>[2x]DADLDKQVNTAGAWPIATGGYYSQHNSPLAQINKSNVKNVKAAWSFSTGVLNGHEGAPLVIGDMMYVHSAFPNNTYALNLNDPGKIVWQHKPKQDASTKAVMCCDVVDRGLAYGAGQIVKKQANGHLLALDAKTGKINWEVEVCDPKVGSTLTQAPFVAKDTVLMGCSGAELGVRGAVNAFDLKTGELKWRAFATGSDDSVRLAKDFNSANPHYGQFGLGTKTWEGDAWKIGGGTNWGWYAYDPKLNLFYYGSGNPAPWNETMRPGDNKWTMTIWGRDLDTGMAKWGYQKTPHDEWDFAGVNQ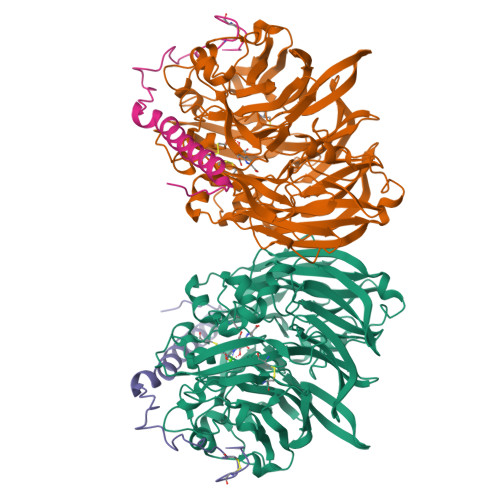MVLTDQPVNGKMTPLLSHIDRNGILYTLNRENGNLIVAEKVDPAVNVFKKVDLKTGTPVRDPEFATRMDHKGTNICPSAMGFHNQGVDSYDPESRTLYAGLNHICMDWEPFMLPYRAGQFFVGATLAMYPGPNGPTKKEMGQIRAFDLTTGKAKWTKWEKFAAWGGTLYTKGGLVWYATLDGYLKALDNKDGKELWNFKMPSGGIGSPMTYSFKGKQYIGSMYGVGGWPGVGLVFDLTDPSAGLGAVGAFRELQNHTQMGGGLMVFSL;>[2x]YDGQNCKEPGNCWENKPGYPEKIAGSKYDPKHDPVELNKQEESIKAMDARNAKRIANAKSSGNFVFDVK> MMINIQEDKLVSAHDAEEILRFFNCHDSALQQEATTLLTQEAHLLDIQAYRAWLEHCVGSEVQYQVISRELRAASERRYKLNEAMNVYNENFQQLKVRVEHQLDPQNWGNSPKLRF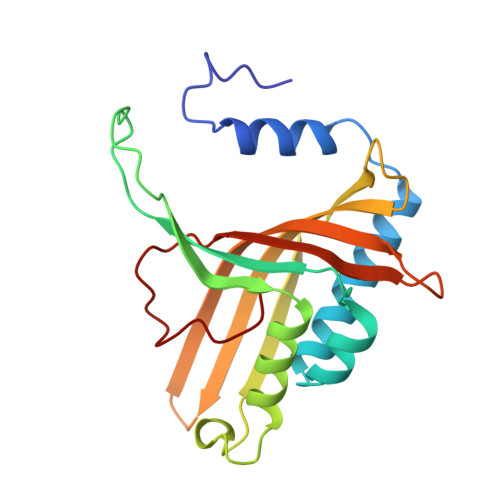TRFITNVQAAMDVNDKELLHIRSNVILHRARRGNQVDVFYAAREDKWKRGEGGVRKLVQRFVDYPERILQTHNLMVFL> PDSLFAGLVGEYYGTNSQLNNISDFRALVDSKEADATFEAANISYGRGSSDVAKGTHLQEFLGSDASTLSTDPGDNTDGGIYLQGYVYLEAGTYNFKVTADDGYEITINGNPVATVDNNQSVYTVTHASFTISESGYQAIDMIWWDQGGDYVFQPTLSADGGSTYFVLDSAILSSTGETPYT

MpPA14 (Marinomonas primoryensis PA14 domain) lectin is a domain of a 1.5-MDa adhesin responsible for a symbiotic bacterium-diatom interaction in Antarctica. Bioinformatic analyses indicated the presence of an ∼20-kDa domain near the C terminus of MpIBP that is a member of the PA14 family, which is a carbohydrate-binding lectin module widely distributed across several kingdoms of life. PA14 domains share a β-sandwich fold and the presence of two consecutive aspartate residues in a cis peptide linkage (DcisD). The DcisD motif coordinates a Ca2+ ion that is directly involved in binding polar vicinal hydroxyl groups of various carbohydrates.

MpPA14 lectin bound l-fucose most strongly, with a Kdapp of 0.65 mM, followed by N-acetylglucosamine (GlcNAc) (Kdapp = 1.07 mM). With Kd values of 147 μM and 170 μM for l-fucose and GlcNAc, these two ligands had a greater than 2-fold higher affinity for MpPA14 than did glucose (Kd = 350 μM). However, the well-resolved 1-Å electron density map in this study unambiguously showed that fucose bound MpPA14 with its cis 3,4-diol in the gauche conformation with a dihedral angle of 47°. In contrast to the MpPA14 hexose ligands, which are all in the d-configuration, fucose is in the l-configuration, with hydroxyl groups of the fucopyranose ring pointed in opposite directions. This helps the endocyclic oxygen atom of fucose point toward L11 and hydrogen bond with the sidechain of Gln156. Additionally, the hydroxyl on the α-anomeric carbon may hydrogen bond with the sidechain of Ser130 on L9, clamping the pyranose ring tightly into the binding site. The l-fucose–MpPA14 interaction is distinct from that shown by the bacterial C-type lectin, LecB, from Pseudomonas aeruginosa, which uses two side-by-side Ca2+ ions to directly coordinate the 2,3,4-triol of l-fucose. The additional ionic interaction between LecB and l-fucose can explain its enhanced affinity (Kd = 58 μM) for the sugar compared to that of MpPA14 (Kd = 147 μM). The addition of 0.5 mM l-fucose was extremely effective at blocking accumulation of lectin on the diatom, as the free sugar outcompeted the cell surface glycans for the binding MpPA14 and displaced 95% of the fluorescent signal.> IDTAALKEEVLKYMNRCSTQDLADMTGCTLAEAEFMVAKRPFPDLESALVVKQPRPVIPKGRRGRREKTPLGPRLVGICMEIMRGYFVVDALIRQCEQLGGKIQRGIEAWGLSNTATSDEGETSLVNFDQMKSFGTPANSSFITTPPASFSPDIKLQDYQIIGINWLYLLYELKLAGILADEMGLGKTCQTIAFFSLLMDKNINGPHLVIAPASTMENWLREFAKFCPKLKIELYYGSQVEREEIRERINSNKDSYNVMLTTYRLAATSKADRLFLRNQKFNVCVYDEGHYLKNRASERYRHLMSIPADFRVLLTGTPLQNNLKELISLLA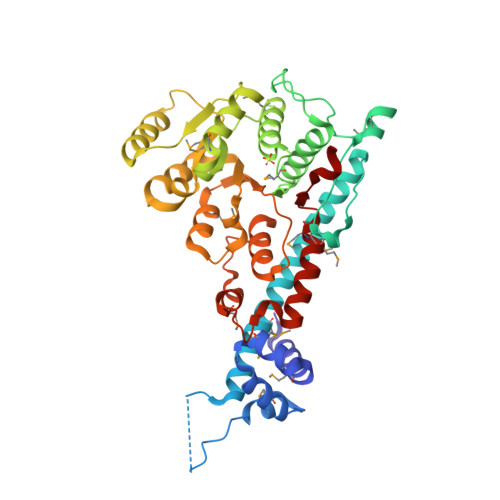FILPHVFDYGLKSLDVIFTMKKSPESDFERALLSEQRVSRAKMMMAPFVLRRKKSQVL> MNARSTGQHPARYPGAAAGEPTLDSWQEPPHNRWAFAHLGEMVPSAAVSRRPVNAPGHALVRLGAIAAQLPDLEQRLEQTYTDAFLVLRGTEVVAEYYRAGFAPDDRHLLMSVSKSLCGTVVGVLVDEGRIDPAQPVTEYVPELAGSVYDGPSVLQVLDMQISIDYNEDYVDPASEVQTHGRSAGWSTRRHGDPADTYEFLTTLRGDGSTGEFQYCSANTDVLAWIVERVTGLRYVEALSTYLWAKLDADRDATITVDTTG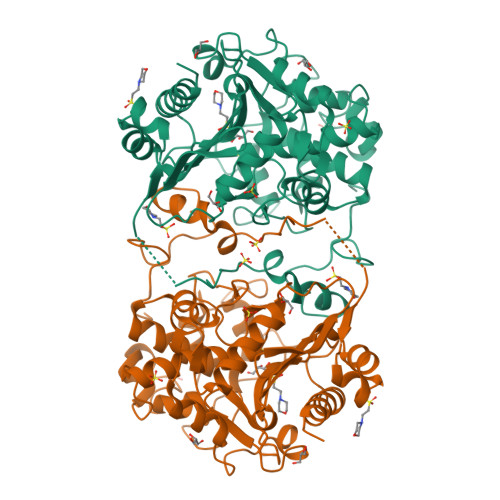FGCAHGGVSCTARDLARVGRMMLDGGVAPRGRVVSEDWVRRVLAGGSHEAMTDKGFTNTFPDGSYTRQWWCTGNERANVSGIGIHGQNLWLDPLTDSVIVKLSSWPDPYTEHWHRLQNGILLDVSRALDAV> MKFTNLTAKEFGAFTDSMPYSHFTQTVGHYELKLAEGYETHLVGIKNNNNEVIAACLLTAVPVMKVFKYFYSNRGPVIDYENQELVHFFFNELSKYVKKHRCLYLHIDPYLPYQYLNHDGEITGNAGNDWFFDKMSNLGFEHTGFHKGFDPVLQIRYHSVLDLKDKTADDIIKNMDGLRKRNTKKVKKNG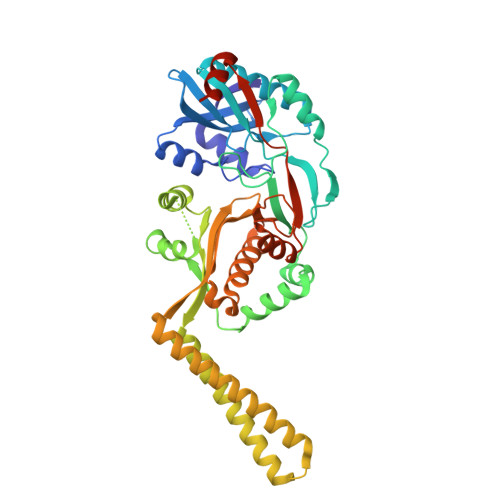VKVRFLSEEELPIFRSFMEDTSESKAFADRDDKFYYNRLKYYKDRVLVPLAYINFDEYIKELNEERDILNKDLNKALKDIEKRPENKKAHNKRDNLQQQLDANEQKIEEGKRLQEEHGNELPISAGFFFINPFEVVYYAGGTSNAFRHFAGSYAVQWEMINYALNHGIDRYNFYGVSGKFTEDAEDAGVVKFKKGYNAEIIEYVGDFIKPINKPVYAAYTALKKVKDRIFHHHHHH(S)-N-(4-carbamimidoylbenzyl)-1-(2-(cyclohexylamino)ethanoyl)pyrrolidine-2-carboxamide 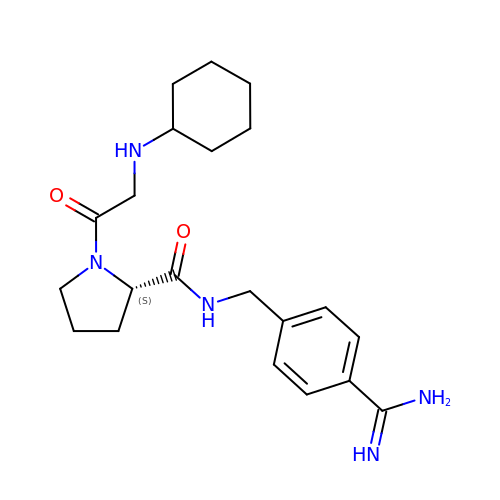| C21 H31 N5 O2 | RYKFVFFOIYLADT-SFHVURJKSA-N>[2x]GVVLYARVSSHDRRSDLDRQVARLTAWATERDLGVGQVVCEVGSGLNGKRPKLRRILSDPDARVIVVEHRDRLARFGVEHLEAALSAQGRRIVVADPGETTDDLVCDMIEVL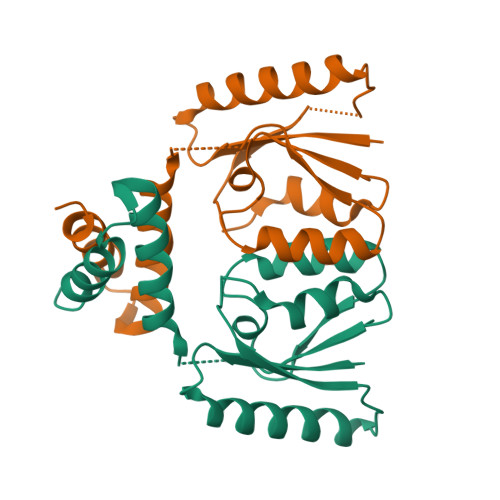TGMCARLYGRRGARNRAMRAVTEAKREPGAG> LYHTVPPAVVGVGGGGVNAGPVASGAIVGTNGYVITTLHSVSKLPEISVQVATTGGIRRFPAQVVKTIPGHDLALLKMQTTEKFLHFRMADVQTVVPGQQVFAFGRNMAGAPLVRQGLVQSADAPLAVGATQITHLLRSDAVYSWEQTGGPLVNAQGDLVGINIAATGPTGKVEGFTVPAQVIVSHLQ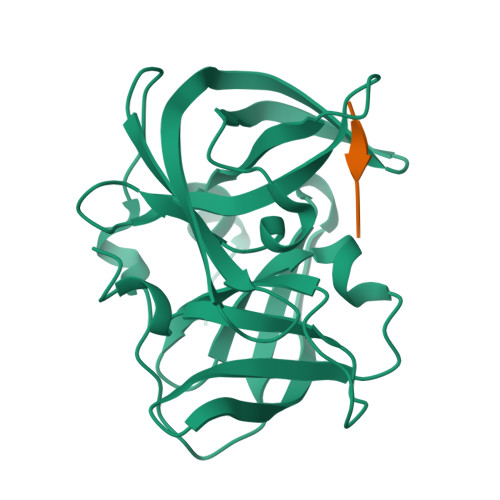D>[4x]GAMAPLQPGDSFPANVVFSYIPPTGSLDLTVSGRPIEYNASEALAKGTSVLVAV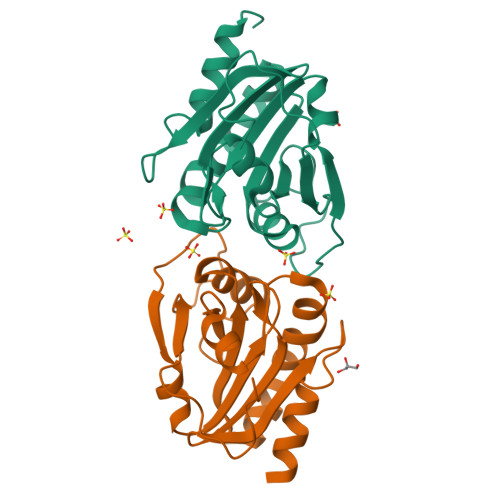PGAFTPTCQEKHVTGFIAKLDQLRQAGVDRVLFIASNDAFVMSAWGKANGIKDESILFLSDSDTAFSSSIGWANAGRTGRYAIVVKDGKVVYAAVDTVRGSTEKSGVDAVLTVLGNQGKL URIDINE-5'-DIPHOSPHATE-N-ACETYLMURAMOYL-L-ALANINE-D-GLUTAMATE | C28 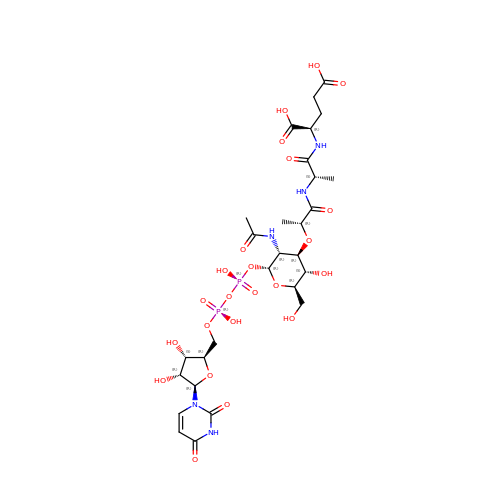H43 N5 O23 P2 | OJZCATPXPWFLHF-HPUCEMLMSA-N> MGPSLDFALSLLRRNVRQVQTDQGHFTMLGVRDRLAVLPRHSQPGKTIWIEHKLVNILDAVELVDEQGVNLELTLITLDTNEKFRDITKFIPENISTASDATLVINTEHMPSMFVPVGDVVQYGFLNLSGKPTHRTMMYNFPTKAGQCGGVV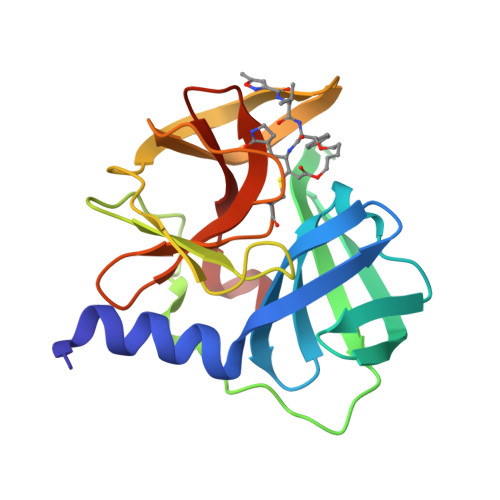TSVGKVIGIHIGGNGRQGFCAGLKRSYFA> MAWNQPGNNGQDRDPWGSSKPGGNSEGNGNKGGRDQGPPDLDDIFRKLSKKLGGLGGGKGTGSGGGSSSQGPRPQLGGRVVTIAAAAIVIIWAASGFYTIKEAERGVVTRFGKFSHLVEPGLNWKPTFIDEVKPV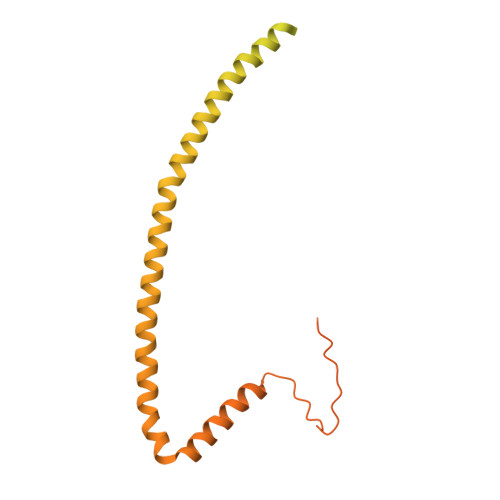NVEAVRELAASGVMLTSDENVVRVEMNVQYRVTNPEKYLYSVTSPDDSLRQATDSALRGVIGKYTMDRILTEGRTVIRSDTQRELEETIRPYDMGITLLDVNFQAARPPEEVKAAFDDAIAARENEQQYIREAEAYTNEVQPRANGQAQRILEEARAYKAQTILEAQGEVARFAKLLPEYKAAPEITRERLYIETMEKVLGNTRKVLVNDKGGNLMVLPLDQMLKGGNAPAAKSDNGASNLLRLPPASSSTTSGASNTSSTSQGDIMDQRRANAQRNDYQRQGE>[4x]MIALIQRVTRASVTVEGEVTGEIGAGLLVLLGVEKDDDEQKANRLCERVLGYRIFSDAEG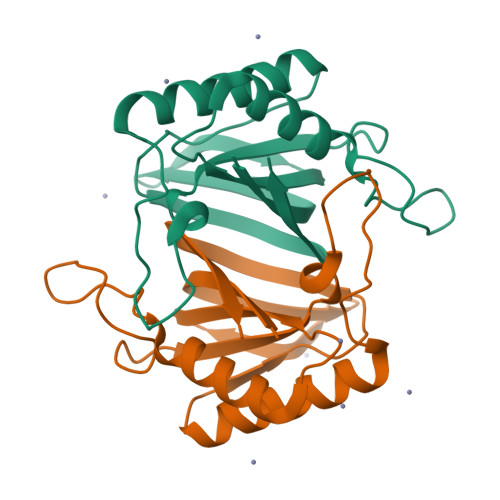KMNLNVQQAGGSVLVVSQFTLAADTERGMRPSFSKGASPDRAEALYDYFVERCRQQEMNTQTGRFAADMQVSLVNDGPVTFWLQV>SMRNVALITGITGQDGSYLAEFLLEKGYEVHGIVRRSSSFNTGRIEHLYKNPQAHIEGNMKLHYGDLTDSTCLVKIINEVKPTEIYNLGAQSHVKISFDLAEYTADVDGVGTLRLLDAVKTCGLINSVKFYQASTSELYGKVQEIPQKETTPFYPRSPYGAAKLYAYWIVVNFREAYNLFAVNGILFNHESPRRGANFVTRKISRSVAKIYLGQLECFSLGNLDAKRDWGHAKDYVEAMWLMLQNDEPEDFVIATGEVHSVREFVEKSFLHIGKTIVWEGKNENEVGRC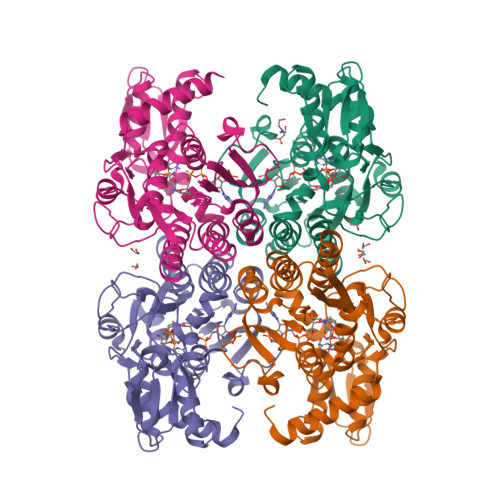KETGKVHVTVDLKYYRPTEVDFLQGDCTKAKQKLNWKPRVAFDELVREMVHADVELMRTNPNA[4x]> MNSNSIQSFDALPHNLRECFLDMASFLEDQRIIASTIIDLWSASYGKEGMNNLQDLASRNLLKLLPIGRNEYEDGFYNELLVKQDNVLREFAINQCLKESSSIFERKRLNLEIQDNKFPNWCLNPKQPIVINASLFSISTDDSFASSWFEMDCPNVEALVLNISSSNYALPNFIATMKELKVVIIINHGLE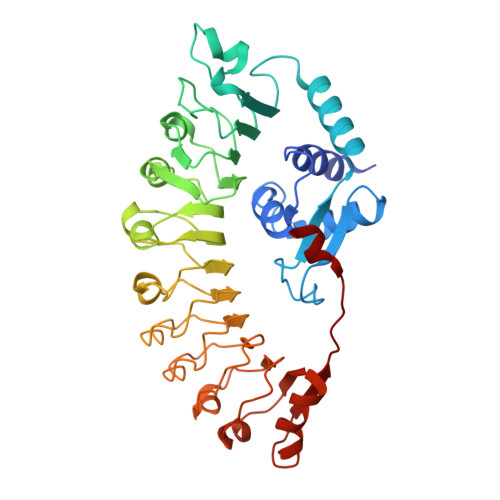PAKLTNLSCLSSLPNLKRIRFEKVSISLLDIPKLGLKSLEKLSLWFCHVVDALNELEDVSETLQSLQEIEIDYCYNLDELPYWISQVVSLKKLSVTNCNKLCRVIEAIGDLRDLETLRLSSCASLLELPETIDRLDNLRFLDVSGGFQLKNLPLEIGKLKKLEKISMKDCYRCELPDSVKNLENLEVKCDEDTAFLWKILKPEMKNLTITEEKTEHNLNLLQLF> MEVNRTVSPNIQTGRKTTNSFLKSILIFTILISSTVLLVGGYWIFKEMAPRPKEVRSESGEVLMTKETIIGGQAVFQKYGLMDYGTVLGHGSYMGPDYTAEALKVYTEGMQDYKAKERYNKPFADLTDDEKSIIREQVIKEMRKNRYNPVTDVLVLTDAQVYGLEKVRDYYRDVFTNGDGWGLKKGLIKESDMPKANRAWVADSDQIQQIADFFFWTAWLSSTLRIG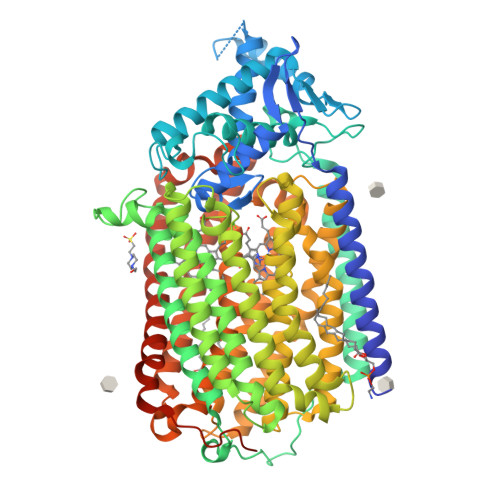DEITYTNNWPYYEDAGNTMSFSAVWWSGASVTILILFIGIILYVFYRYQLSMQEAYAEGKFPVIDLRRQPLTPSQVKAGKYFVVVSALFFVQTMFGALLAHYYTEPDSFFGINWIYDILPFNIAKGYHLQLAIFWIATAWLGMGIFIAPLVGGQEPKKQGLLVDLLFWALVVLVGGSMIGQWLGVNGYLGNEWFLLGHQGWEYIELGRIWQIILVVGMLLWLFIVFRGVKRGLKRESDKGGLIHLLFYSAIAVPFFYIFAFFIQPDTNFTMADFWRWWIIHLWVEGIFEVFAVVVIGFLLVQLRLVTKKSTVRALYFQFTILLGSGVIGIGHHYYYNGSPEVWIALGAVFSALEVIPLTLLILEAYEQYKMMRDGGANFPYKATFWFLISTAIWNLVGAGVFGFLINLPAVSYFEHGQFLTPAHGHAAMMGVYGMFAIAVLLYSLRNIVKPEAWNDKWLKFSCWMLNIGLAGMVVITLLPVGILQMKEAFIHGYWASRSPSFLQQDVVQNLLLVRAVPDTIFLIGVVALLVFAIKALFHLRKPTHGEGEELPVANHWMKDRLKNSLEHHHHHH The yeast eisosome, composed of the BAR-domain proteins Pil1 and Lsp1 (hereafter, Pil1/Lsp1), scaffolds a membrane compartment that senses and responds to mechanical stress by flattening and releasing sequestered factors. MCC–eisosomes are relatively stable, and have been implicated in sensing and responding to plasma membrane stress: various stimuli, including hypo-osmotic shock, heat shock and mechanical pressure, cause eisosomes to flatten and release sequestered proteins to affect signalling or transport functions. Here we isolated near-native eisosomes as helical tubules made up of a lattice of Pil1/Lsp1 bound to plasma membrane lipids, and solved their structures by helical reconstruction.

We isolated MCC–eisosomes from S. cerevisiae using a gentle purification procedure, preserving a lattice of untagged Pil1/Lsp1 structural proteins bound to a presumably intact plasma membrane bilayer in a near-native state, observable as a two-layer density in the protein tubule. Although MCC–eisosomes have been shown to have a furrow-like half-pipe structure in vivo, our isolated eisosome tubules seem to be closed, continuous helices of Pil1/Lsp1 proteins. Using a symmetry expansion and density subtraction strategy, we could refine our structures to a resolution of around 3.2 Å, which allowed us to build models of the paralogues Pil1 and Lsp1. With our improved resolution, we could characterize the lattice contact sites between Pil1 dimers in detail. Two novel structured regions of the protein were visible in our maps: (1) a folded N terminus (Nt) that forms lattice contact sites with the Nt of a neighbouring dimer, followed by (2) an Nt amphipathic helix (AH; residues 39–48) buried within the lipid density of the cytoplasmic leaflet of the bilayer that runs parallel to the BAR-domain helices of each Pil1/Lsp1 monomer. By making one-pixel slices through the unsharpened maps parallel to the axis of the eisosome tubule, we could clearly see the well-defined protein density of the AH buried in the cytoplasmic leaflet of the membrane, which is visible in these images as a uniform density of lower intensity (teal arrow). At slices around 5 Å deeper, an array of small voids in the membrane density begins to appear just below the AH. This pattern continues throughout the cytoplasmic leaflet, producing a fence-like striation in the membrane (violet arrows). Visualization of the electrostatic surface on the membrane-facing surface of the Pil1 dimer revealed two patches of intense positive charge adjacent to the AHs.

>MHRTYSLRNSRAPTASQLQNPPPPPSTTKGRFFGKGGLAYSFRRSAAGAFGPELSRKLSQLVKIEKNVLRSMELTANERRDAAKQLSIWGLENDDDVSDITDKLGVLIYEVSELDDQFIDRYDQYRLTLKSIRDIEGSVQPSRDRKDKITDKIAYLKYKDPQSPKIEVLEQELVRAEAESLVAEAQLSNITRSKLRAAFNYQFDSIIEHSEKIALIAGYGKALLELLDDSPVTPGETRPAYDGYEASKQIIIDAESALNEWTLDSAQVKPTLSFKQDYEDFEPEEGEEEEEEDGQGRWSEDEQEDGQIEEPEQEEEGAVEEHEQVGHQQSESLPQQTTA[14x]> MPLPKTHELHIFGSFNGVKFDMVGEGTGNPNEGSEELKL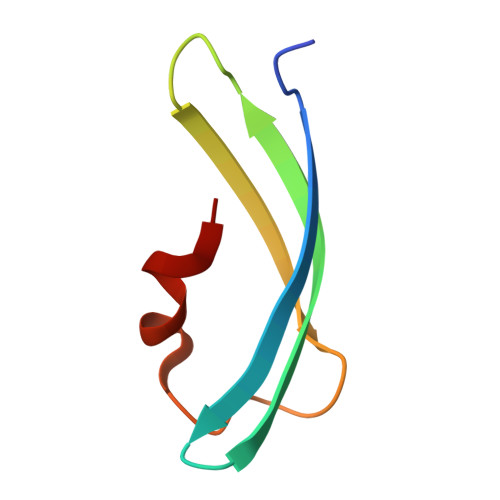KSTNGPLKFSPYILVPHLG> GPMPGKKVVARV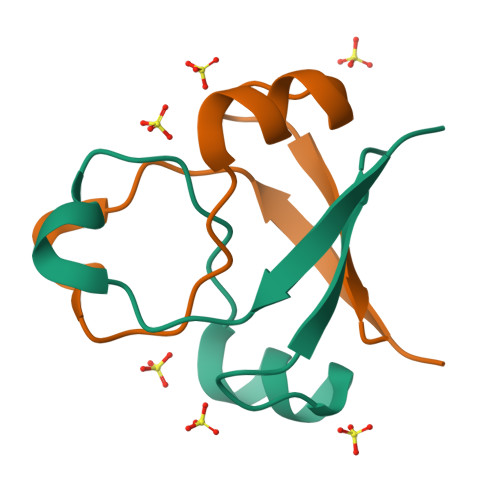AEARAEDVGKRVVRVDKAERAKVGVKVGDVVEVKKV> IRNTNEYTEGPTV;> GSLIGLMKDAFQPHHHHHHHLSPHPPGTVDKKMVEKCWKLMDKVVRLCQNPKLALKNSPPYILDLLPDTYQHLRTILSRYEGKMETLGENEYFRVFMENLMKKTKQTISLFKEGKERMYEENSQPRRNLTKLSLIFSHMLAELKGIFPSGLFQGDTFRITKADAAEFWRKAFGEKTIVPWKSFRQALHEVHPISSGLEAMALKSTIDLTCNDYISVFEFDIFTRLFQPWSSLLRNWNSLAVTHPGYMAFLTYDEVKARLQKFIHKPGSYIFRLSCTRLGQWAIGYVTADGNILQTIPHN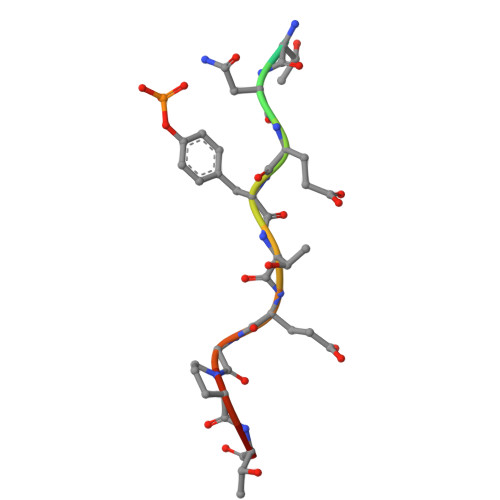KPLFQALIDGFREGFYLFPDGRNQNPDLTG>MTTTSNSTETGRRPGRLGDPDRCLRTDPRTDPRTVEALAPFGLDVNAAPAPIGPDAPREQQLEYAMGAEAAFEGVFAALMDGLDPVPGIERRTETISGPAGNEIKLYVHRPAGAVGPLPGIFHIHGGGMVILQAAGPVYVRFRDELAATGTVVVGVEYRNGAGVLGPHPFPAGLHDCAVALDWVHARRAELGISTLTVAGESGGGNLTLATAIRAKREGRLDAIDGVYALVPYISGMYGRSREEREAELPSLVECDGYFISCDLCA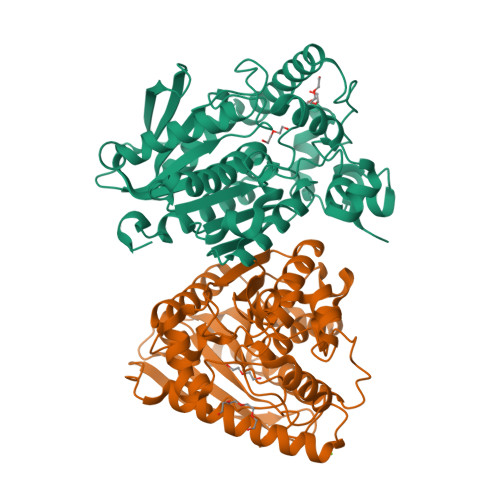VFVEVYDPGTAHLTDPLAWPYHAAREDLVGLPPHVISVNEVDPLRDEGLAYYRKLVEAGVEARSRVVPGACHAADMMFRKAAPDMYEATVQDIHDFVTSLHRLEHHHHHH[2x]> GAMKTVGYAIVGTGYFGAELGRIMKEQEGARIVAVLDPENGQTIAEELDCDVETDLDTLYSREDVEAVIVATPNYLHKEPVIKAAEHGVNVFCEKPIALSYQDCDEMVRTCQEHGVIFMAGHVMNFFHGVRYAKKLINDGVIGKVLYCHSARNGWEEQQPTISWKKIREKSGGHLYHHIHELDCVQFLMGGMPEEVTMTGGNVAHQGEAFGDEDDMLFVNMQFSDNRYAVLEWGSAFHWPEHYVLIQGTKGAIKIDMCDCGGTLKVDGREEHFLVHESQEEDDDRTRIYHGTEMDGAIMYGKPGKKPPMWLHSIMKNEMKYLNGILHGKEVDDEFRPLLTGEAARAAIATADACTKSRFEDRKVKLSEIIGEGS;> MKTVGYAIVGTGYFGAELGRIMKEQEGARIVAVLDPENGQTIAEELDCDVETDLDTLYSREDVEAVIVATPNYLHKEPVIKAAEHGVNVFCEKPIAL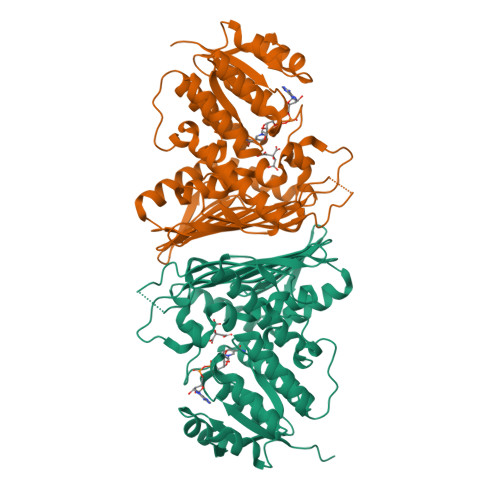SYQDCDEMVRTCQEHGVIFMAGHVMNFFHGVRYAKKLINDGVIGKVLYCHSARNGWEEQQPTISWKKIREKSGGHLYHHIHELDCVQFLMGGMPEEVTMTGGNVAHQGEAFGDEDDMLFVNMQFSDNRYAVLEWGSAFHWPEHYVLIQGTKGAIKIDMCDCGGTLKVDGREEHFLVHESQEEDDDRTRIYHGTEMDGAIMYGKPGKKPPMWLHSIMKNEMKYLNGILHGKEVDDEFRPLLTGEAARAAIATADACTKSRFEDRKVKLSEIIG> DEQPEPRTRRRAYLWCKEFLPGAWRGLREDEFHISVIRGGLSNMLFQCSLPDTTATLGDEPRKVLLRLYGAILQMRSCNKEGSEQAQKENEFQGAEAMVLESVMFAILAERSLGPKLYGIFPQGRLEQFIPSRRLDTEELSLPDISAEIAEKMATFHGMKMPFNKEPKWLFGTMEKYLKEVLRIKFTEESRIKKLHKLLSYNLPLELENLRSLLESTPSPVVFCHNDCQEGNILLLEGRENSEKQKLMLIDFEYSSYNYRGFDIGNHFCEWMYDYSYEKYPFFRANIRKYPTKKQQLHFISSYLPAFQNDFENLSTEEKSIIKEEMLLEVNRFALASHFLWGLWSIVQAKISSIEFGYMDYAQARFDAYFHQKRKLGV

The synthesis is initiated by phosphorylation of Cho and Etn to render phosphocholine (PCho) and phosphoethanolamine (PEtn) by choline kinase (CK) and ethanolamine kinase (EK) respectively. In humans, CK is encoded by two genes, which express three isoforms CKα1, CKα2 and CKβ. An overexpression of the α-isoform of CK has been identified as an oncogene that mediates human cell transformation. As with many of the kinases that initiate the Kennedy pathway, the HsCKα1 is able to phosphorylate both Cho and Etn12.

Only crystals of HsCKα1 in complex with compound BR25 were obtained that enabled us to solve the structure and unambiguously interpret the electron density maps. As expected, the crystal structure shows that BR25 is located within the known Cho-binding site. Strikingly the compound favors the unusual conformation also found for BR33 in which a new adjacent binding site is formed that is located at the back of the Cho-binding site. Whereas compounds adopting the typical binding mode contain a short and rigid linker consisting of a biphenyl group, BR25 and BR33 have the flexible linker 1,4-biphenylbutane, explaining why the latter compounds adopt the unusual binding mode in which the aperture of an adjacent binding site is induced. Compound BR25, in contrast to compound BR23, induces local conformational changes of several amino acids, allowing the 4-(dimethylamino)pyridinium fragment to access the adjacent binding site. This is mainly evidenced by W420 in which a dramatic conformational change occurs. The rest of BR25 is located in the Cho-binding site. The two positively charged fragments of BR25 forces the molecule to adopt a twisted conformation to maximize their interactions with the enzyme. While the 4-(dimethylamino)pyridinium fragment is characterized by a parallel π-cation interaction with Y333 and W420, respectively, the 4-pyrrolidinopyridinium fragment is tethered by Y354, W420, F435 and Y440.> MADQENSPLHTVGFDARFPQQNQTKHCWQSYVDYHKCVNMKGEDFAP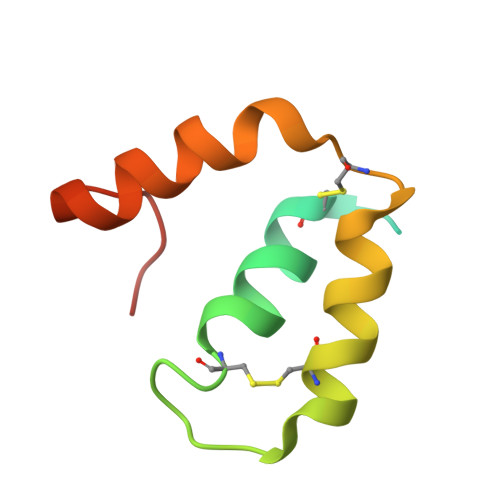CKVFWKTYNALCPLDWIEKWDDQREKGIFAGDINSD>[7x]AEPVYPDQLRLFSLGQGVCGDKYRPVNREEAQSV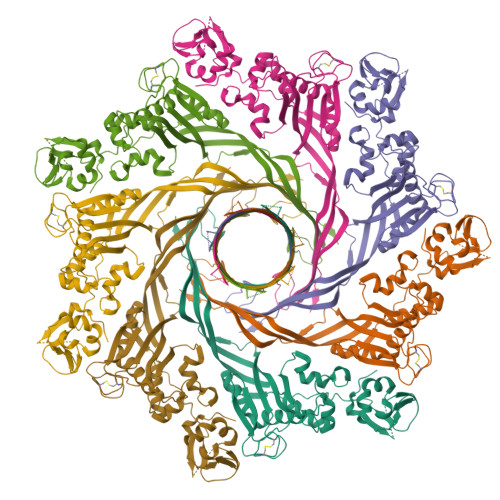KSNIVGMMGQWQISGLANGWVIMGPGYNGEIKPGTASNTWCYPTNPVTGEIPTLSALDIPDGDEVDVQWRLVHDSANFIKPTSYLAHYLGYAWVGGNHSQYVGEDMDVTRDGDGWVIRGNNDGGCDGYRCGDKTAIKVSNFAYNLDPDSFKHGDVTQSDRQLVKTVVGWAVNDSDTPQSGYDVTLRYDTATNWSKTNTYGLSEKVTTKNKFKWPLVGETALSIAIAANQSWASQNGGSTTTSLSQSVRPTVPARSKIPVKIELYKADISYPYEFKADVSYDLTLSGFLRWGGNAWYTHPDNRPNWNHTFVIGPYKDKASSIRYQWDKRYIPGEVKWWDWNWTIQQNGLSTMQNNLARVLRPVRAGITGDFSAESQFAGNIEIGAPVPLAA>MGRDPNSTNDTTTQNVVLTKYGFDKDVTAIDRATDQIWTGDGAKPLQGVDFTIYNVTA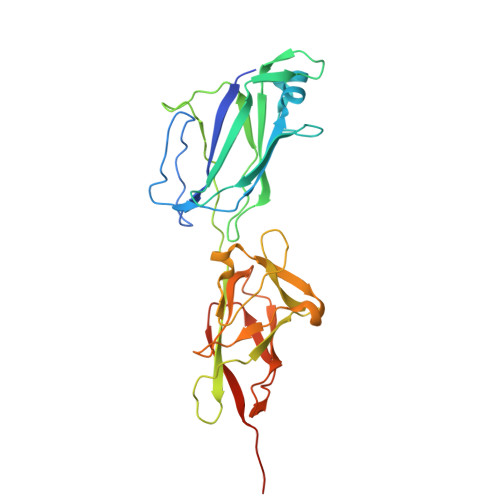NYWASPKDYKGSFDSAPVAATGTTNDKGQLTQALPIQSKDASGKTRAAVYLFHETNPRAGYNTSADFWLTLPAKAAADGNVYVYPKNVQKTTYERTFVKKDAETKEVLEGAGFKISNSDGKFLKLTDKDGQSVSIGEGFIDVLANNYRLTWVAESDATVFTSDKSGKFGLNGFADNTTTYTAVETNVPDGYDAAANTDFKADNSSSDILDAPSGILPLEHHHHHH[3x]>[4x]MNPNQKIITIGSVSLTIATVCFLMQIAILATTVTLHFKQHECDSPASNQVMPCEPIIIERNITEIVYLNNTTIEKEICPKVVEYRNWSKPQCQITGFAPFSKDNSIRLSAGGDIWVTREPYVSCDPGKCYQFALGQGTTLDNKHSNDTVHDRIPHRTLLMNELGVPFHLGTRQVCIAWSSSSCHDGKAWLHVCITGDDKNATASFIYDGRLVDSIGSWSQNILRTQESECVCINGTCTVVMTDGSASGRADTRILFIEEGKIVHISPLSGSAQHIEECSCYPRYPGVRCICRDNWKGSNRPVVDINMEDYSIDSSYVCSGLVGDTPRNDDSSSNSNCRNPNNERGTQGVKGWAFDNGNDLWMGRTISKESRSGYETFKVIGGWSTPNSKSQVNRQVIVDNNNWSGYSGIFSVEGKSCINRCFYVELIRGRPQETRVWWTSNSIVVFCGTSGTYGTGSWPDGANINFMPI

NA, which is a sialidase, catalyzes hydrolysis of terminally linked sialic acid and functions as the receptor-destroying element of influenza A and B viruses. Additionally, influenza A NA is further classified into two groups: group 1 (N1, N4, N5 and N8) and group 2 (N2, N3, N6, N7 and N9), based upon primary sequence. Group 1 NAs contain a 150-cavity (formed by amino acids 147–151 of the 150-loop) in their active site, whereas group 2 NAs lack this cavity. NA inhibition assays were carried out and complex crystal structures were solved for laninamivir, laninamivir octanoate, zanamivir and oseltamivir in order to elucidate the structural basis of their inhibition.

Laninamivir octanoate complex structures with p09N1 and p57N2 were solved at 1.6 Å and 2.2 Å, respectively, demonstrating that the laninamivir octanoate prodrug can also directly inhibit NA without further processing. Furthermore, we confirm the binding of the prodrug, laninamivir octanoate, to p57N2, with a similar binding mode to laninamivir. The complex structure of p57N2 with the laninamivir octanoate prodrug has a similar binding mode to laninamivir and zanamivir, however laninamivir octanoate in complex with p09N1 is completely different. Additionally, p57N2 Arg224 forms a unique hydrogen bond with the laninamivir octanoate 9-ester carbonyl, and p09N1 Asn294 and Ser247 form unique hydrogen bonds with the laninamivir octanoate 9-ester-O. However, the novel conformation of the laninamivir octanoate-p09N1 complex disrupts any hydrogen bonding with Glu276. ***The laninamivir octanoate 9-ester-carbonyl forms a hydrogen bond with N2 Arg224. The native His274 is also further away from Glu276 in our p57N2-laninamivir octanoate structure and does not hydrogen bond with it. In both structures, there is no observed electron density corresponding to the octanoyl carbon chain indicating that this part of the molecule is highly flexible and does not engage many stable hydrophobic interactions with p09N1 or p57N2. The disordered octanoyl carbon chain likely destabilizes the interactions between the NA active site and the laninamivir octanoate 8-OH and 9-ester, which is indicated by the lower electron density surrounding the 9-ester. Hence inhibition of p57N2 by laninamivir octanoate was much better than for p09N1. The overall lack of hydrogen bonds and instability in the p09N1-laninamivir octanoate structure relative to p57N2 provides the structural basis for higher laninamivir octanoate inhibition of p57N2 observed in our study and a previous report demonstrating better laninamivir octanoate inhibition of H2N2 and H3N2 viruses over H1N1 viruses.>[8x]MVPTQAHPEWYKSAVFYELSVRTFQDGNGDGKGDFPGLTSRLDYLKNLGVDCLWLLPWFPSPLRDDGYDVADYRGIHPDLGTLDDFKVFLREAHARGLWVIGDLVTNHTSSDHPWFQAARRGPTLPDGSPNEYHDYYVWSDEGKEYADTRIIFTDTEVSNWTLDEQAGKYYWHRFFASQPDLNYDNPKVVEELHGAARFWLDLGLDGFRVDAVPYLIEREGTSCENLPETHEILKGFRAMVDREYPGRLLLAEANQWPEEVVEYFGTEAEPEFHMCFNFPVMPRLYMSLKREDTSSIREIMGRLPKIPSFGQWCIFLRNHDELTLEMVTDDE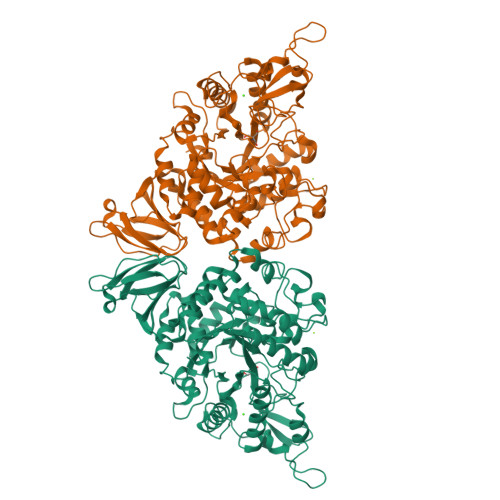RAFMYAAYAPDARMKINVGIRRRLAPLLDNDRRRIELLNTVLLALPGSPVLYYGDEIGMGDDLGLPDRNGVRTPMQWNAGTSGGFSTAQPSDCFFPPIQDPVYGFGRVNVQSQLQDPSSLLKWTARQLELRRAHPAFAHGDLTFIETGNPAILAFTRQYDGETLLIVSNFAGNAQAGLLDLAPFVGRAPVTLSGASPLPVVTGNGQYPVVMGKYDYYWLRLNSRVDKLAAALEHHHHHH> MGSLVCVGTGLQLAGQISVLSRSYIEHADIVFSLLPDGFSQRWLTKLNPNVINLQQFYAQNGEVKNRRDTYEQMVNAILDAVRAGKKTVCALYGHPG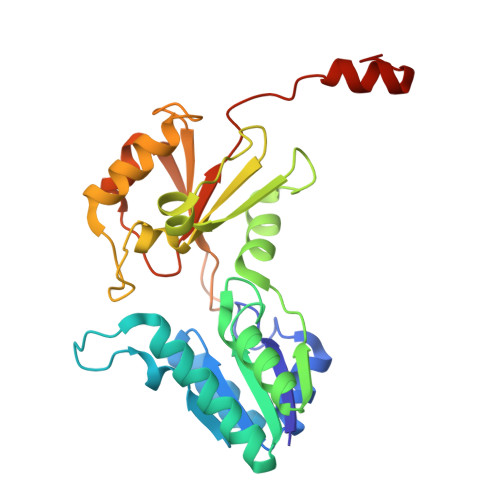VFACVSHMAITRAKAEGFSAKMEPGISAEACLWADLGIDPGNSGHQSFEASQFMFFNHVPDPTTHLLLWQIAIAGEHTLTQFHTSSDRLQILVEQLNQWYPLDHEVVIYEAANLPIQAPRIERLPLANLPQAHLMPISTLLIPPAKKLEYNYAILAKLGIGPEDLG>GAKQLSTARKFKMITGKDLFQQQKA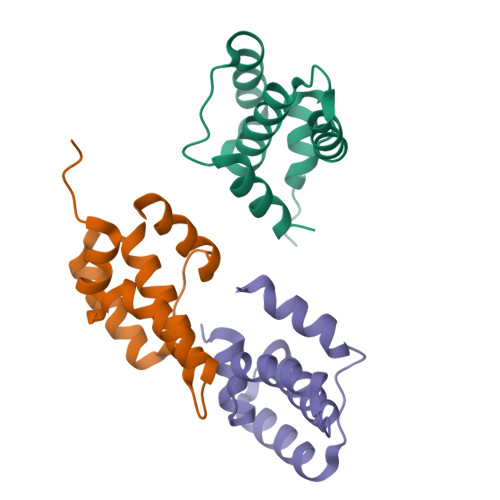MDTELKKEDGEITDLMEFVQYGLYLALFQDNIVKAKSDFSDFRSSFEFDTDGKGLKELVELWQKEI[3x]>[8x]MKNNGGARVVVIGAGFVGASYVFALMNQGIADEIVLIDANESKAIGDAMDFNHGKVFAPKPVDIWHGDYDDCRDADLVVICAGANQKPGETRLDLVDKNIAIFRSIVESVMASGFQGLFLVATNPVDILTYATWKFSGLPHERVIGSGTILDTARFR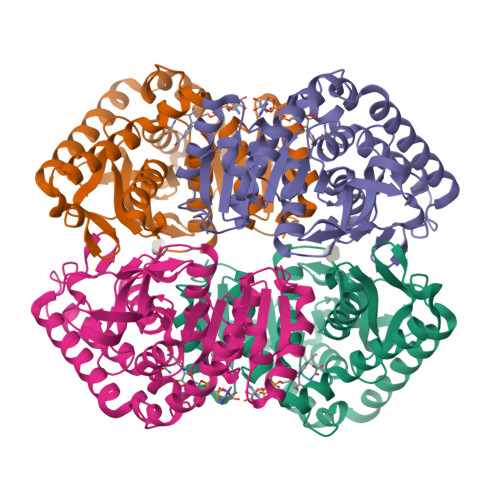FLLGEYFSVAPQNVHAYIIGEHGDTELPVWSQAYIGVMPIRKLVESKGEEAQKDLERIFVNVRDAAYQIIEKKGATYYGIAMGLARVTRAILHNENAILTVSAYLDGLYGERDVYIGVPAVINRNGIREVIEIELNDDEKNRFHHSAATLKSVLARAFT L-XYLITOL 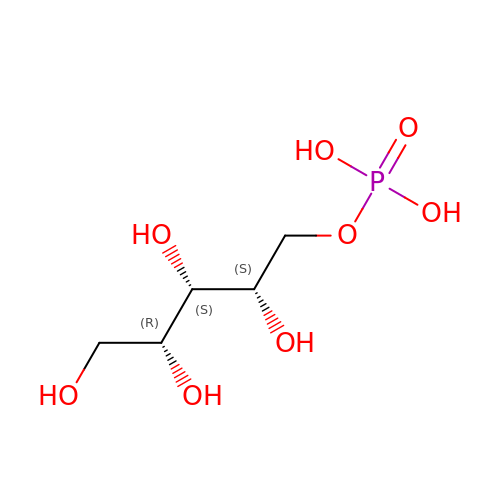5-PHOSPHATE | C5 H13 O8 P | VJDOAZKNBQCAGE-WISUUJSJSA-N> IWELKKDVYVVELDWYPDAPGEMVVLTCDTPEEDGITWTLDQSSEVLGSGKTLTIQVKEFGDAGQYTCHKGGEVLSHSLLLLHKKEDGIWSTDILKDQKEPKNKTFLRCEAKNYSGRFTCWWLTTISTDLTFSVKSSRGSSDPQGVTCGAATLSAERVRGDNKEYEYSVECQEDSACPAAEESLPIEVMVDAVHKLKYENYTSSFFIRDIIKPDPPKNLQLKPLKNSRQVEVSWEYPDTWSTPHSYFSLTFCVQVQGKSKREKKDRVFTDKTSATVICRKNASISVRAQDRYYSSSWSEWASVPCS;> RAVPGGSSPAWTQCQQLSQKLCTLAWSAHPLVGHMDLREEGDEETTNDVPHIQCGDGCDPQGLRDNSQFCLQRIHQGLIFYEKLLGSDIFTGEPSLLPDSPVGQLH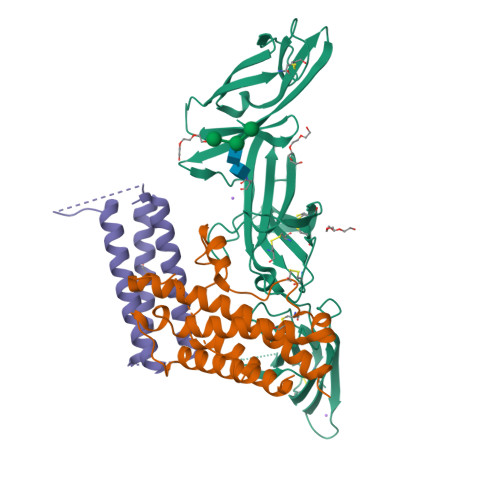ASLLGLSQLLQPEGHHWETQQIPSLSPSQPWQRLLLRFKILRSLQAFVAVAARVFAHGAATLSPGTKHHHHHH;> HMSIQEIQKEIAQIQAVIAGIQKYIYTMTGGSGGSGGGGSGGSGGMSIEEIQKQIAAIQCQIAAIQKQIYAMTGSGGGGSGGSGGGGSGMSIEEIQKQIAAIQEQILAIYKQIMAMVT>[10x]MAYRKRGARRETNLKQDDRMQEKEENKNVNTNSENKNATKPQLSEKVLSQKEEVITDNQEEIKIADEVKKSNKEESKQLLEVLKTKEEHQKEVQYEILQKTIPTFEPKESILKKLEDIKPEQVKKQTKLFRIFEPRQLPVYRANGEKELRNRWYWKLKRDTLPDGDYDVREYFLNLYDQVLTEMPDYLLLKDMAVENKNSRDAGKVVDSETAAICDAIFQDEETEGVVRRFIAEMRQRVQADRNVVNYPSILHPIDHAFNEYFLQHQLVEPLNNDIIFNYIPERIRNDVNYILNMDRNLPSTARYIRPNLLQDRLNLHDNFESLWDTITTSNYILARSVVPDLKELVSTEAQIQKMSQDLQLEALTIQSETQFLTGINSQAANDCFKTLIAAMLSQRTMSLDFVTTNYMSLISGMWLLTVVPNDMFIRESLVACQLAIINTIIYPAFGMQRMHYRNGDPQTPFQIAEQQIQNFQVANWLHFVNNNQFRQVVIDGVLNQVLNDNIRNGHVVNQLMEALMQLSRQQFPTMPVDYKRSIQRGILLLSNRLGQLVDLTRLLAYNYETLMACITMNMQHVQTLTTEKLQLTSVTSLCMLIGNATVIPSPQTLFHYYNVNVNFHSNYNERINDAVAIITAANRLNLYQKKMKSIVEDFLKRLQIFDISRVPDDQMYRLRDRLRLLPVEIRRLDIFNLILMNMEQIERASDKIAQGVIIAYRDMQLERDEMYGYVNIARNLDGFQQINLEELMRTGDYAQITNMLLNNQPVALVGALPFITDSSVISLVAKLDATVFAQIVKLRKVDTLKPILYKINSDSNDFYLVANYDWVPTSTTKVYKQIPQQFDFRASMHMLTSNLTFTVYSDLLAFVSADTVEPINAVAFDNMRIMNEL;> MGKYNLILSEYLSFIYNSQS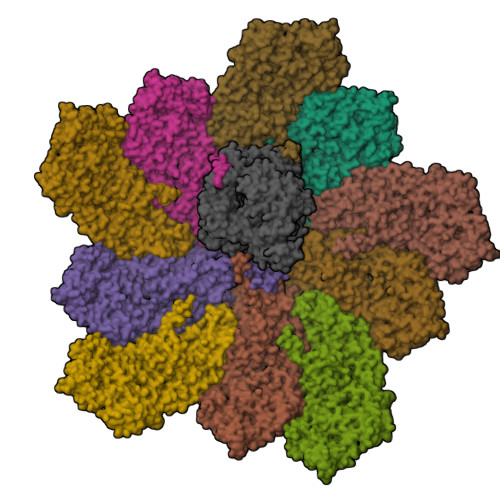AVQIPIYYSSNSELENRCIEFHSKCLENSKNGLSLKKLFVEYSDVIENATLLSILSYSYDKYNAVERKLVKYAKGKPLEADLTVNELDYENNKITSELFPTAEEYTDLLMDPAILTSLSSNLNAVMFWLEKHENDVAEKLKIYKRRLDLFTIVASTVNKYGVPRHNAKYRYEYEVMKDKPYYLVTWANSSIEMLMSVFSHEDYLIARELIVLSYSNRSTLAKLVSSPMSILVALVDINGTFITNEELELEFSNKYVRAIVPDQTFDELKQMLDNMRKAGLTDIPKMIQDWLVDCSIEKFPLMAKIYSWSFHVGFRKQKMLDAALDQLKTEYTEDVDDEMYREYTMLIRDEVVKMLEEPVKHDDHLLQDSELAGLLSMSSASNGESRQLKFGRKTIFSTKKNMHVMDDMANGRYTPGIIPPVNVDKPIPLGRRDVPGRRTRIIFILPYEYFIAQHAVVEKMLIYAKHTREYAEFYSQSNQLLSYGDVTRFLSNNSMVLYTDVSQWDSSQHNTQPFRKGIIMGLDMLANMTNDARVIQTLNLYKQTQINLMDSYVQIPDGNVIKKIQYGAVASGEKQTKAANSIANLALIKTVLSRISNKYSFATKIIRVDGDDNYAVLQFNTEVTKQMVQDVSNDVRETYARMNTKVKALVSTVGIEIAKRYIAGGKIFFRAGINLLNNEKKGQSTQWDQAAVLYSNYIVNRLRGFETDREFILTKIMQMTSVAITGSLRLFPSERVLTTNSTFKVFDSEDFIIEYGTTDDEVYIQRAFMSLSSQKSGIADEIAASSTFKNYVSRLSEQLLFSKNNIVSRGIALTEKAKLNSYAPISLEKRRAQISALLTMLQKPVTFKSSKITINDILRDIKPFFTVNEAHLPIQYQKFMPTLPDNVQYIIQCIGSRTYQIEDDGSKSAISRLISKYSVYKPSIEELYKVISLHENEIQLYLISLGIPKIDADTYVGSKIYSQDKYRILESYVYNLLSINYGCYQLFDFNSPDLEKLIRIPFKGKIPAVTFILHLYAKLEVINHAIKNGSWISLFCNYPKSEMIKLWKKMWNITSLRSPYTNANFFQD> NEAIECHLSDLLQQLTSVNASKPSERGLVRQEEAEDPACIPIFWVSKWVDYSDKYGLGYQLCDNSVGVLFNDSTRLILYNDGDSLQYIERDGTESYLTVSSHPNSLMKKITLLNYFRNYMSEHLLKAGANITPREGDELARLPYLRTWFRTRSAIILHLSNGTVQINFFQDHTKLILCPLMAAVTYINEKRDFQTYRLSLLEEYGCCKELASRLRYARTMVDKLLSSRSASNRLKAS;> SPLVTSTIKTEDVVSNSQNSRLHFSQHKTSTI

One of CSFs, Emi2 (also known as F-box only protein 43) inhibits APC/C activity by binding to APC/C-cdc20; therefore, Emi2 blocks the ubiquitin-mediated proteolysis of MPF8910. Subsequently, the phosphorylated threonines in Emi2 can be recognized by Plk1, which undergoes phosphorylation, and these phosphorylated sites serve as a recognition site for SCF, another class of ubiquitin ligases; SCF destabilizes Emi2 and activates APC/C10. In this study, one of our aim was to elucidate recognition of Emi2 by the Polo-box domain (PBD) of Plk1 using X-ray crystallography and biochemical characterization. To elucidate the detailed molecular mechanism of recognition of Emi2 by Plk1-PBD, we determined structure of the complexes of PBD domain (367–603 of Plk1) with peptides Emi2146–177 or Emi2169–177.

We synthesized two phosphothreonine-containing peptides spanning the amino acid positions 146–177 and 169–177 of Emi2, where two threonines (Thr152 and Thr176) were phosphorylated, and their binding affinity for Plk1-PBD was measured by isothermal titration calorimetry (ITC). The peptide Emi2146–177, which contains phospho-Thr152 and phospho-Thr176, showed higher binding affinity (Kd = 1.73 μM) than did the peptide 169–177 (which has a single phosphothreonine: Thr176), which had a Kd value of 29.58 μM. ITC results suggested that the phosphopeptide 146–177 can bind to two Plk1-PBDs simultaneously (n = 0.47, expressed as a ratio of Emi2146–177 to Plk1-PBD), whereas phosphopeptide 169–177 binds an equimolar amount of Plk1-PBD (n = 0.92, expressed as a ratio of Emi2169–177 to Plk1-PBD). When a threefold excess of Plk1-PBD was mixed with Emi2146–177, most of Plk1 was eluted in peaks corresponding to 60 kDa. These results show that both phosphothreonine-containing motifs near Thr152 or Thr176 can recruit Plk1-PBD. First, we crystallized Plk1-PBD with Emi2146–177, which has two phosphothreonine residues (Thr152 and Thr176) and solved the complex’s structure at 2.4 Å. Although ITC and SEC-MALS indicated that the phosphorylated Emi2146–177 peptides can bind two PBDs simultaneously, only one binding event between the PBD and a phosphopeptide observed in an asymmetric unit in the crystal structure. We examined the structure of the Plk1-PBD·Emi2146–177 complex containing various complexes of Plk1-PBD with cdc25 originated peptide or chemical 4j, and we found that Emi2′s peptide-binding characteristics in relation to Plk1-PBD are similar to those previously reported for phosphopeptides (especially closely related to the Plk1-cdc25c structure). One considerable difference with the previous findings in the complex of Plk1-PBD with Emi2146–177 is that the extra electron density corresponds to Asp157, Val158, and Val159 bound to a negatively charged surface patch of Plk1-PBD (left in circle). In addition, the negatively charged patch interacts with Asp157, Val158, and Val159 of Emi2, which also lie in the conserved region.>[2x]PHI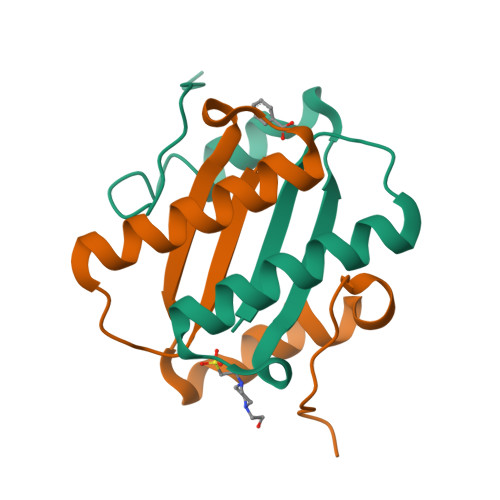DIKCFPRELDEQQKAALAADITDVIIRHLNSKDSSISIALQQIQPESWQAIWDAEIAPQMEALIKKPGYSMNA> SMEFQAALSRKVAELVHFLLLKYRAREPVT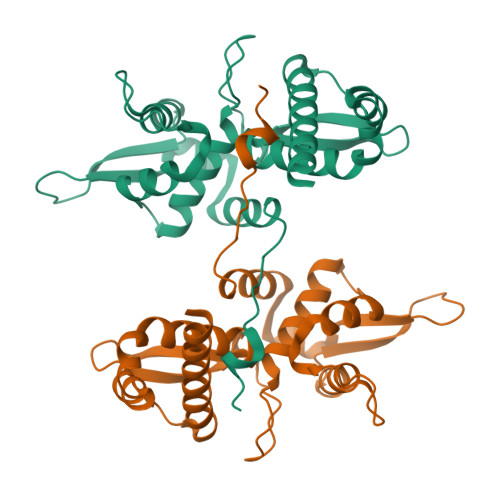KAEMLGSVVGNWQYFFPVIFSKASSSLQLVFGIELMEVDPIGHLYIFATCLGLSYDGLLGDNQIMPKAGLLIIVLAIIAREGDCAPEEKIWEELSVLEVFEGREDSILGDPKKLLTQHFVQENYLEYRQVPGSDPACYEFLWGPRALVETSYVKVLHHMVKISGGPHISYPPLHEWVLREGEE>CGTATATACG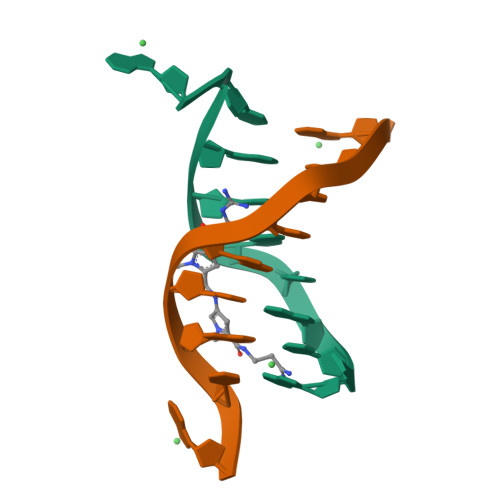[2x]>[4x]MGAHSKEMAPLMGKRTTAPGGNPVVLTEKRPADLTPTKKSAHFFLEIEGFEPNPTVTKTSPPIFSKPMDSNIRQCLSGNCDDMDSPQSPQDDVTETPSNPNSPSANLAKEEQRQKKKRLKKRIFAAVSEGCVEELRELLQDLQDLCRRRRGLDVPDFLMHKLTASDTGKTCLMKALLNINPNTKEIVRILLAFAEENDILDRFINAEYTEEAYEGQTALNIAIERRQGDITAVLIAAGADVNAHAKGVFFNPKYQHEGFYFGETPLALAACTNQPEIVQLLMENEQTDITSQDSRGNNILHALVTVAEDFKTQNDFVKRMYDMILLRSGNWELETMRNNDGLTPLQLAAKMGKAEILKYILSREIKEKPLRSLSRKFTDWAYGPVSSSLYDLTNVDTTTDNSVLEIIVYNTNIDNRHEMLTLEPLHTLLHTKWKKFAKYMFF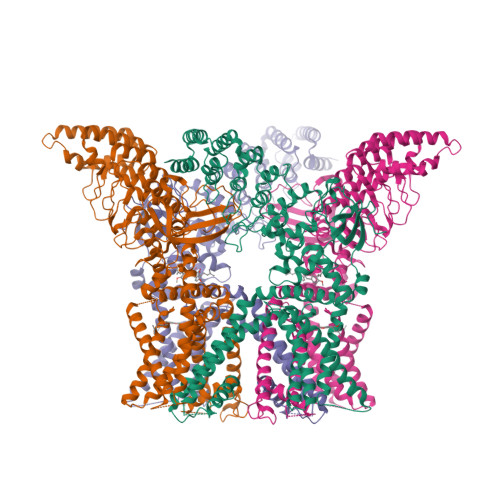LSFCFYFFYNITLTLVSYYRPREDEDLPHPLALTHKMSWLQLLGRMFVLIWATCISVKEGIAIFLLRPSDLQSILSDAWFHFVFFVQAVLVILSVFLYLFAYKEYLACLVLAMALGWANMLAYTRGFQSMGMYSVMIQKVILHDVLKFLFVYILFLLGFGVALASLIEKCSKDKKDCSSYGSFSDAVLELFKLTIGLGDLNIQQNSTYPILFLFLLITYVILTFVLLLNMLIALMGETVENVSKESERIWRLQRARTILEFEKMLPEWLRSRFRMGELCKVADEDFRLCLRINEVKWTEWKTHVSFLNEDPGPIRRTADLNKIQDSSRSNSKTTLYAFDELDEFPETSVLVPRGSAAAWSHPQFEK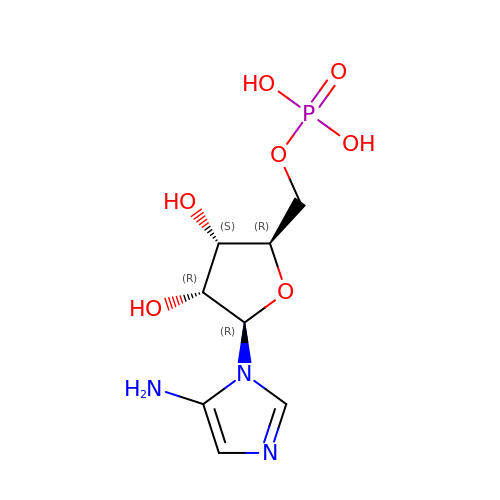5-AMINOIMIDAZOLE RIBONUCLEOTIDE | C8 H14 N3 O7 P | PDACUKOKVHBVHJ-XVFCMESISA-N>SSKQKVDLQSLPTRAYLDQTVVPILLQGLAVLAKERPPNPIEFLASYLLKNKAQFEDRNLERPHRD[4x];> NTLDTLYKEQIAEDIVWDIIDELEQIALQQ

From yeast to mammals, the SET1 and MLL-like (mixed-lineage leukemia) multi-subunit protein complexes, known as SET1 or MLL COMPASS, are responsible for H3K4 methylation. Dpy30 is an important subunit of MLL/SET1 complexes, where it plays an essential role in both catalyzing H3K4 trimethylation and maintaining the state of trimethylated H3K4. Dpy30 directly interacts with Ash2L in human (Bre2 in yeast) COMPASS through its Dpy30-binding motif (DBM). Although the structures of the human Dpy30 C-terminal domain (Dpy30C) and SPRY domain of Ash2L containing the DBM motif were solved, the binding mode and stoichiometry of Dpy30 and Ash2L within COMPASS remain uncertain, partly because the complex structure is lacking.

However, the complex of Dpy30C and Bre2DBM was crystallized successfully and the structure (Dpy30C-Bre2DBM) was solved to 2.15 Å resolution. The crystal structure of Dpy30C-Bre2DBM contains two dimers of Dpy30C (chain A and B: AB dimer; chain C and D: CD dimer) and only one copy of Bre2DBM (chain E) in an asymmetrical unit. Finally, two separated structures, with the orientation of the helix different from each other, were refined and showed similar qualities with Rwork/Rfree of 0.18/0.21 and 0.18/0.22, respectively. It is likely that the structure represents a mixed model, which was led by the fact that some DBM helices were bound in one orientation and the rest were in a reversed orientation in the complex crystal. In the two types of structures, the DBM peptide interacts with Dpy30C in the same mode and position, although in opposite orientation. The Bre2DBM peptide interacts simultaneously with two Dpy30C dimers, albeit with different affinities. The CD dimer plays a dominant role in Bre2DBM binding with a buried area of about 836.2 Å2, while the AB dimer assists in the interaction, forming a binding area of about 292.5 Å2 with Bre2. The interactions between Dpy30C and Bre2DBM are mainly hydrophobic without specific hydrogen-bond or salt-bond interactions. Ten hydrophobic residues from chains C and D of the Dpy30C dimer are distributed symmetrically on the inner surface in a semi-circular shape, forming a hydrophobic groove. In the Dpy30-Bre2DBM complex structure, two Dpy30 dimers form a loose tetramer with a crossing angle of 60°. Bre2DBM binding to Dpy30C increases this area to 1128.7 Å2, which stabilizes the Dpy30C tetramer. This structure represents a model of Dpy30 binding to the target helix at the ratio of 4:1.> MDNVLPVDSDLSPNISTNTSEPNQFVQPAWQIVLWAAAYTVIVVTSVVGNVVVMWIILAHKRMRTVTNYFLVNAAFAEASMAAFNTVVNFTYAVHNEWYYGLFYCKFHNFFPIAAIFASIYSMTAVAFDRYMAIIHPLQPRLSLTATKVVICVIWVLALLLAFPQGYYSTTETMPSRVVCKIEWPEHPNKIYEKVYHICVTVLIYFLPLLVIGYLYTVVGITLRASGIDCSFWNESYLTGSRDERKKSLLSKFGMDEGVTFMFIGRFDRGQKGVDVLLKAIEILSSKKEFQEMRFIIIGKGDPELEGWARSLEEKHGNVKVITEMLSREFVRELYGSVDFVIIPSYFEPFGLVALEAMCLGAIPIASAVGGLR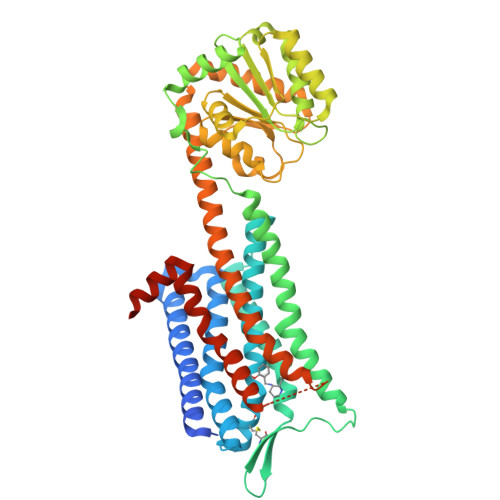DIITNETGILVKAGDPGELANAILKALELSRSDLSKFRENCKKRAMSFSEQVSAARKVVKMMIVVVCTFAICWLPFHIFFLLPYINPDLYLKKFIQQVYLAIMWLAMSSTMYNPIIYCCLNDRFRLGFKHAFRCCPFISAGDYEGLE>[2x]GSLHMSFETRFEKMDNLLRDPKSEVNSDCLLDGLDALVYDL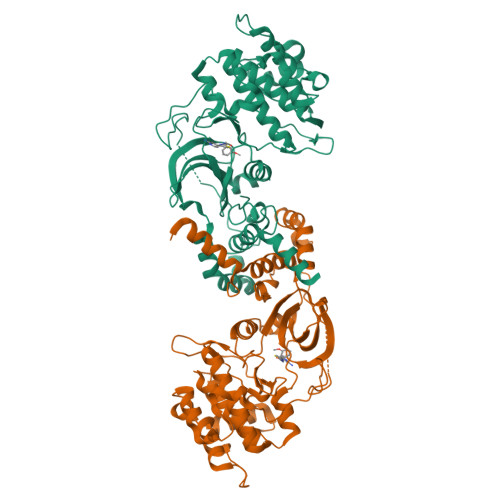DFPALRKNKNIDNFLSRYKDTINKIRDLRMKAEDYEVVKVIGRGAFGEVQLVRHKSTRKVYAMKLLSKFEMIKRSDSAFFWEERDIMAFANSPWVVQLFYAFQDDRYLYMVMEYMPGGDLVNLMSNYDVPEKWARFYTAEVVLALDAIHSMGFIHRDVKPDNMLLDKSGHLKLADFGTCMKMNKEGMVRCDTAVGTPDYISPEVLKSQGGDGYYGRECDWWSVGVFLYEMLVGDTPFYADSLVGTYSKIMNHKNSLTFPDDNDISKEAKNLICAFLTDREVRLGRNGVEEIKRHLFFKNDQWAWETLRDTVAPVVPDLSSDIDTSNFDDLEEDKGEEETFPIPKAFVGNQLPFVGFTYYSNRRYLSSANPNDNR>[4x]MAEALFKEIDVNGDGAVSYEEVKAF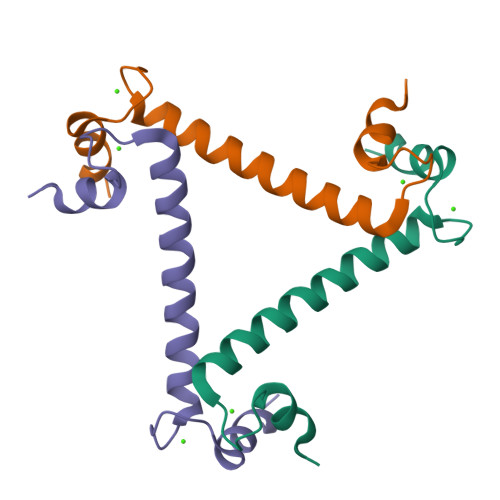VSKKRAIKNEQLLQLIFKSIDADGNGEIDQNEFAKFYGSIQ> MKPEVEQELAHILLTELLAYQFASPVRWIETQDVFLKDFNTERVVEIGPSPTLAGMAQRTLKNKYESYDAALSLHREILCYSKDAKEIYYTPDPSELAAKEEPAKEEAPAPTPAASAPAPAAAAPAPVAAAAPAAAAAEIADEPVKASLLLHVLVAHKLKKSLDSIPMSKTIKDLVGGKSTVQNEILGDLGKEFGTTPEKPEETPLEELAETFQDTFSGALGKQSSSLLSRLISSKMPGGFTITVARKYLQTRWGLPSGRQDGVLLVALSNEPAARLGSEADAKAFLDSMAQKYASIVGVDLSSAASASGAAGAGAAAGAAMIDAGALEEITKDHKVLARQQLQVLARYLKMDLDNGERKFLKEKDTVAELQAQLDYLNAELGEFFVNGVATSFSRKKARTFDSSWNWAKQSLLSLYFEIIHGVLKNVDREVVSEAINIMNRSNDALIKFMEYHISNTDETKGENYQLVKTLGEQLIENCKQVLDVDPVYKDVAKPTGPKTAIDKNGNITYSEEPREKVRKLSQYVQEMALGGPITKESQPTIEEDLTRVYKAISAQADKQDISSSTRVEFEKLYSDLMKFLESSKEIDPSQTTQLAGMDVEDALDKDSTKEVASLPNKSTISKTVSSTIPRETIPFLHLRKKTPAGDWKYDRQLSSLFLDGLEKAAFNGVTFKDKYVLITGAGKGSIGAEVLQGLLQGGAKVVVTTSRFSKQVTDYYQSIYAKYGAKGSTLIVVPFNQGSKQDVEALIEFIYDTEKNGGLGWDLDAIIPFAAIPEQGIELEHIDSKSEFAHRIMLTNILRMMGCVKKQKSARGIETRPAQVILPMSPNHGTFGGDGMYSESKLSLETLFNRWHSESWANQLTVCGAIIGWTRGTGLMSANNIIAEGIEKMGVRTFSQKEMAFNLLGLLTPEVVELCQKSPVMADLNGGLQFVPELKEFTAKLRKELVETSEVRKAVSIETALEHKVVNGNSADAAYAQVEIQPRANIQLDFPELKPYKQVKQIAPAELEGLLDLERVIVVTGFAEVGPWGSARTRWEMEAFGEFSLEGCVEMAWIMGFISYHNGNLKGRPYTGWVDSKTKEPVDDKDVKAKYETSILEHSGIRLIEPELFNGYNPEKKEMIQEVIVEEDLEPFEASKETAEQFKHQHGDKVDIFEIPETGEYSVKLLKGATLYIPKALRFDRLVAGQIPTGWNAKTYGISDDIISQVDPITLFVLVSVVEAFIASGITDPYEMYKYVHVSEVGNCSGSGMGGVSALRGMFKDRFKDEPVQNDILQESFINTMSAWVNMLLISSSGPIKTPVGACATSVESVDIGVETILSGKARICIVGGYDDFQEEGSFEFGNMKATSNTLEEFEHGRTPAEMSRPATTTRNGFMEAQGAGIQIIMQADLALKMGVPIYGIVAMAATATDKIGRSVPAPGKGILTTAREHHSSVKYASPNLNMKYRKRQLVTREAQIKDWVENELEALKLEAEEIPSEDQNEFLLERTREIHNEAESQLRAAQQQWGNDFYKRDPRIAPLRGALATYGLTIDDLGVASFHGTSTKANDKNESATINEMMKHLGRSEGNPVIGVFQKFLTGHPKGAAGAWMMNGALQILNSGIIPGNRNADNVDKILEQFEYVLYPSKTLKTDGVRAVSITSFGFGQKGGQAIVVHPDYLYGAITEDRYNEYVAKVSAREKSAYKFFHNGMIYNKLFVSKEHAPYTDELEEDVYLDPLARVSKDKKSGSLTFNSKNIQSKDSYINANTIETAKMIENMTKEKVSNGGVGVDVELITSINVENDTFIERNFTPQEIEYCSAQPSVQSSFAGTWSAKEAVFKSLGVKSLGGGAALKDIEIVRVNKNAPAVELHGNAKKAAEEAGVTDVKVSISHDDLQAVAVAVSTKK;> MDAYSTRPLTLSHGSLEHVLLVPTASFFIASQLQEQFNKILPEPTEGFAADDEPTTPAELVGKFLGYVSSLVEPSKVGQFDQVLNLCLTEFENCYLEGNDIHALAAKLLQENDTTLVKTKELIKNYITARIMAKRPFDKKSNSALFRAVGEGNAQLVAIFGGQGNTDDYFEELRDLYQTYHVLVGDLIKFSAETLSELIRTTLDAEKVFTQGLNILEWLENPSNTPDKDYLLSIPISCPLIGVIQLAHYVVTAKLLGFTPGELRSYLKGATGHSQGLVTAVAIAETDSWESFFVSVRKAITVLFFIGVRCYEAYPNTSLPPSILEDSLENNEGVPSPMLSISNLTQEQVQDYVNKTNSHLPAGKQVEISLVNGAKNLVVSGPPQSLYGLNLTLRKAKAPSGLDQSRIPFSERKLKFSNRFLPVASPFHSHLLVPASDLINKDLVKNNVSFNAKDIQIPVYDTFDGSDLRVLSGSISERIVDCIIRLPVKWETTTQFKATHILDFGPGGASGLGVLTHRNKDGTGVRVIVAGTLDINPDDDYGFKQEIFDVTSNGLKKNPNWLEEYHPKLIKNKSGKIFVETKFSKLIGRPPLLVPGMTPCTVSPDFVAATTNAGYTIELAGGGYFSAAGMTAAIDSVVSQIEKGSTFGINLIYVNPFMLQWGIPLIKELRSKGYPIQFLTIGAGVPSLEVASEYIETLGLKYLGLKPGSIDAISQVINIAKAHPNFPIALQWTGGRGGGHHSFEDAHTPMLQMYSKIRRHPNIMLIFGSGFGSADDTYPYLTGEWSTKFDYPPMPFDGFLFGSRVMIAKEVKTSPDAKKCIAACTGVPDDKWEQTYKKPTGGIVTVRSEMGEPIHKIATRGVMLWKEFDETIFNLPKNKLVPTLEAKRDYIISRLNADFQKPWFATVNGQARDLATMTYEEVAKRLVELMFIRSTNSWFDVTWRTFTGDFLRRVEERFTKSKTLSLIQSYSLLDKPDEAIEKVFNAYPAAREQFLNAQDIDHFLSMCQNPMQKPVPFVPVLDRRFEIFFKKDSLWQSEHLEAVVDQDVQRTCILHGPVAAQFTKVIDEPIKSIMDGIHDGHIKKLLHQYYGDDESKIPAVEYFGGESPVDVQSQVDSSSVSEDSAVFKATSSTDEESWFKALAGSEINWRHASFLCSFITQDKMFVSNPIRKVFKPSQGMVVEISNGNTSSKTVVTLSEPVQGELKPTVILKLLKENIIQMEMIENRTMDGKPVSLPLLYNFNPDNGFAPISEVMEDRNQRIKEMYWKLWIDEPFNLDFDPRDVIKGKDFEITAKEVYDFTHAVGNNCEDFVSRPDRTMLAPMDFAIVVGWRAIIKAIFPNTVDGDLLKLVHLSNGYKMIPGAKPLQVGDVVSTTAVIESVVNQPTGKIVDVVGTLSRNGKPVMEVTSSFFYRGNYTDFENTFQKTVEPVYQMHIKTSKDIAVLRSKEWFQLDDEDFDLLNKTLTFETETEVTFKNANIFSSVKCFGPIKVELPTKETVEIGIVDYEAGASHGNPVVDFLKRNGSTLEQKVNLENPIPIAVLDSYTPSTNEPYARVSGDLNPIHVSRHFASYANLPGTITHGMFSSASVRALIENWAADSVSSRVRGYTCQFVDMVLPNTALKTSIQHVGMINGRKLIKFETRNEDDVVVLTGEAEIEQPVTTFVFTGQGSQEQGMGMDLYKTSKAAQDVWNRADNHFKDTYGFSILDIVINNPVNLTIHFGGEKGKRIRENYSAMIFETIVDGKLKTEKIFKEINEHSTSYTFRSEKGLLSATQFTQPALTLMEKAAFEDLKSKGLIPADATFAGHSLGEYAALASLADVMSIESLVEVVFYRGMTMQVAVPRDELGRSNYGMIAINPGRVAASFSQEALQYVVERVGKRTGWLVEIVNYNVENQQYVAAGDLRALDTVTNVLNFIKLQKIDIIELQKSLSLEEVEGHLFEIIDEASKKSAVKPRPLKLERGFACIPLVGISVPFHSTYLMNGVKPFKSFLKKNIIKENVKVARLAGKYIPNLTAKPFQVTKEYFQDVYDLTGSEPIKEIIDNWEKYEQSHHHHHH

Enzymes responsible for synthesis of the lipid precursor palmitate, a 16-carbon chain hydrocarbon molecule, are collectively known as fatty acid synthases (FAS) and are conserved from bacteria to humans. On the other hand, type I FAS, found in actinobacteria and eukaryotes, is an ‘associated system’ where all essential enzymes are expressed by one or two genes and organized into a large, multi-functional assembly line. Substrate and reaction intermediates are shuttled between catalytic centers via a flexibly tethered acyl carrier protein (ACP) domain. In fungi, one or two genes encode all the essential catalytic domains and additional segments that serve as structural domains, stabilizing the assembly into a barrel shaped D3 symmetric dodecamer of ~2.6 megadalton in size.

To our surprise, inactivation of FAS at DH in the presence of substrates resulted in strong cryoEM densities in proximity to the catalytic cavities of the DH domains. Iterative refinement with D3 symmetry applied resulted in a 4.4 Å resolution map of the mutant FAS with improved density for ACP at the stalled DH site. We used the cryoEM density of the truncated model at 15 Å as the initial reference for 3D classification, which was limited to five 3D classes. This resulted in one class with strong ACP density for the shuttling domain that represented ~35% of the symmetry-expanded particle images. Local refinement demonstrated a global resolution of 5.8 Å. The quality of the ACP density was sufficient to allow confident fitting of six out of eight α-helices of the ACP including all four α-helices of the catalytic lobe. Therefore, the observed ACP position is in range for catalysis by the DH domain. The N and C termini of ACP face away from the reaction cavity of the DH domain. This model indicates that both the structural and the canonical lobes of ACP form transient contacts with the chamber scaffold with primarily polar and charged residues lining the interface. Further focused 3D classification in Relion 3.0 on this occupied class demonstrated the conformational heterogeneity of ACP docked at the stalled DH site representing a wobbling motion of the ACP between the ER and the DH domains. The interaction interface of ACP with the DH domain covers a larger surface area and involves multiple structural elements contributed by both the DH and the ER domains. Therefore, when one of the DH sites is occupied by an ACP domain the adjacent ER of the same β-chain protomer is blocked for optimal ACP binding by the other two shuttling domains within the reaction chamber.Kinetoplastid RNA (kRNA) editing takes place in the mitochondria of kinetoplastid protists and creates translatable mRNAs by uridine insertion/deletion. TbRGG2 is a 330 residue protein and contains two main domains, an N-terminal glycine (Gly)-rich region composed of GWG and RG repeats and a C-terminal RNA recognition motif (RRM). Unlike these editing accessory proteins, the T. bruceiRGG2 (TbRGG2) protein is required for editing all nine pan-edited mRNAs. TbRGG2 binds RNA and modulates RNA structure and these functionalities have been shown to be to be essential for its role in kRNA editing.

However, TbRGG2 does not contain the signature aromatic residues within its predicted RRM RNA binding motifs, raising the possibility that it may not adopt a canonical RRM fold. To address this question we determined crystal structures of the domain, which encompasses residues 203 to 269, from the T. brucei protein. Two apo RRM structures were obtained, one of the RRM(L209M) mutant, which was constructed to aid in crystallographic phasing and one of the WT RRM. Both structures were solved to 1.8 Å to final Rwork/Rfree values of 15.1%/18.7% and 16.5%/19.7%, respectively. The WT RRM structure contains four subunits in the crystallographic asymmetric unit (ASU) and the RRM(L209M) structure contains one. The RRM molecules in the two structures are essentially identical; the Cα atoms of the RRM in both structures can be superimposed with root mean square deviations (rmsds) of 0.4–0.6 Å. The structure shows that the TbRGG2 RRM indeed harbors the characteristic RRM fold composed of a five-stranded anti-parallel β-sheet surrounded by two α-helices (36–37). The TbRGG2 RRM structures revealed no interfaces significant enough to provide stable oligomerization, suggesting the domain itself does not oligomerize. Although the TbRGG2 RRM adopts an RRM fold, as noted it does not contain the conserved aromatic residues located on the RNP motifs, characteristic of canonical RRM proteins. Instead it harbors valine, arginine and glutamine residues in these positions.

>GSHMRVQVSGLSDETTWHTLKDHLRQAGEVTFCKVFSGGRAVVEFVTPEDAARAITELQASELEGATLFLR[4x]> MEHVAFGSEDIENTLAKMDDGQLDGLAFGAIQLDGDGNILQYNAAEGDITGRDPKQVIGKNFFKDVAPCTDSPEFYGKFKEGVASGNLNTMFEYTXDYQMTPVKVKVHMKKALSGDSYWVF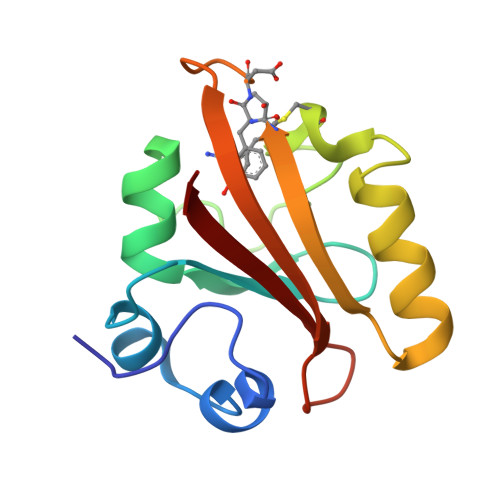VKRV> MTHGAVKTYGIRLRVWGDYACFTRPEMKVERVSYDVMPPSAARGILEAIHWKPAIRWIVDRIHVLRPIVFDNVRRNEVSSKIPKPNPATAMRDRKPLYFLVDDGSNRQQRAATLLRNVDYVIEAHFELTDKAGAEDNAGKHLDIFRRRARAGQSFQQPCLGCREFPASFELLEGDVPLSCYAGEKRDLGYMLLDIDFERDMTPLFFKAVMEDGVITPPSRTSPEVRA;>[7x]MTAIANRYEFVLLFDVENGNPNGDPDAGNMPRIDPETGHGLVTDVCLKRKIRNHVALTKEGAERFNIYIQEKAILNETHERAYTACDLKPEPKKLPKKVEDAKRVTDWMCTNFYDIRTFGAVMTTEVNCGQVRGPVQMAFARSVEPVVPQEVSITRMAVTTKAEAEKQQGDNRTMGRKHIVPYGLYVAHGFISAPLAEKTGFSDEDLTLFWDALVNMFEHDRSAARGLMSSRKLIVFKHQNRLGNAPAHKLFDLVKVSRAEGSSGPARSFADYAVTVGQAPEGVEVKEML;> MILQALHGYYQRMSADPDAGMPPYGTSMENISFALVLDAKGTLRGIEDLREQEGKKLRPRKMLVPIAEKKGNGIKPNFLWENTSYILGVDAKGKQERTDKCHAAFIAHIKAYCDTADQDLAAVLQFLEHGEKDLSAFPVSEEVIGSNIVFRIEGEPGFVHERPAARQAWANCLNRREQGLCGQCLITGERQKPIAQLHPSIKGGRDGVRGAQAVASIVSFNNTAFESYGKEQSINAPVSQEAAFSYVTALNYLLNPSNRQKVTIADATVVFWAERSSPAEDIFAGMFDPPSTTAKPESSNGTPPEDSEEGSQPDTARDDPHAAARMHDLLVAIRSGKRATDI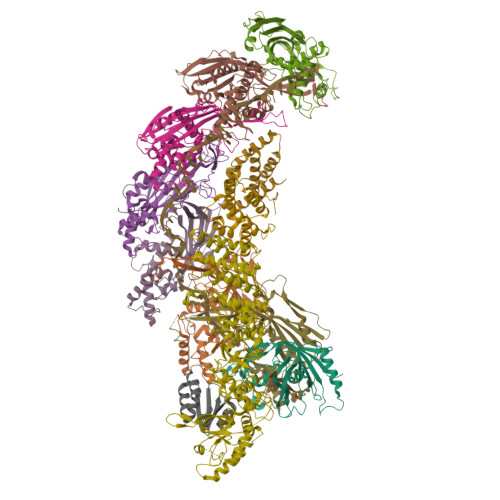MPDMDESVRFHVLGLSPNAARLSVRFWEVDTVGHMLDKVGRHYRELEIIPQFNNEQEFPSLSTLLRQTAVLNKTENISPVLAGGLFRAMLTGGPYPQSLLPAVLGRIRAEHARPEDKSRYRLEVVTYYRAALIKAYLIRNRKLEVPVSLDPARTDRPYLLGRLFAVLEKAQEDAVPGANATIKDRYLASASANPGQVFHMLLKNASNHTAKLRKDPERKGSAIHYEIMMQEIIDNISDFPVTMSSDEQGLFMIGYYHQRKALFTKKNKEN;>[2x]VSLDPARTDRPYLLGRLFAVLEKAQEDAVPGANATIKDRYLASASANPGQVFHMLLKNASNHTAKLRKDPERKGSAIHYEIMMQEIIDNISDFPVTMSSDEQGLFMIGYYHQRKALFTKKNKEN;> MIAQQHKDTVAACEAAEAIAIAKDQVWDGEGYTKYTFDDNSVLIQSGTTQYAMDADDADSIKGYADWLDDEARSAEASEIERLLESVEEE> HHHHHHSEMTPREIVSELDKHIIGQDNAKRSVAIALRNRWRRMQLNEELRHEVTPKNILMIGPTGVGKTEIARRLAKLANAPFIKVEATKFTEVGYVGKEVDSIIRDLTDAAVKMVRVQAIEKNRYRAEELAEERILDVLIPPAKNNWGQTEQQQEPSAARQAFRKKLREGQLDDKEIEIDLAAAPMGVEIMA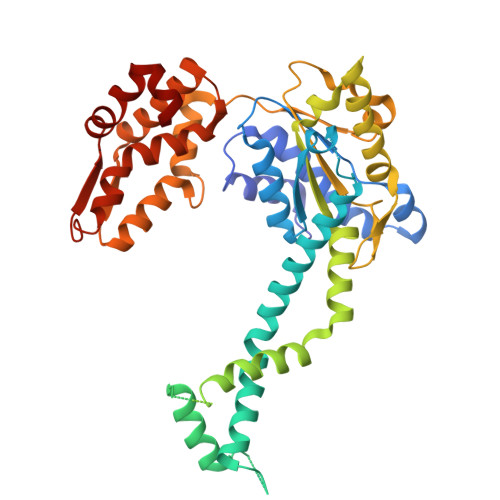PPGMEEMTSQLQSMFQNLGGQKQKARKLKIKDAMKLLIEEEAAKLVNPEELKQDAIDAVEQHGIVFIDQIDKICKRGESSGPDVSREGVQRDLLPLVEGCTVSTKHGMVKTDHILFIASGAFQIAKPSDLIPELQGRLPIRVELQALTTSDFERILTEPNASITVQYKALMATEGVNIEFTDSGIKRIAEAAWQVNESTENIGARRLHTVLERLMEEISYDASDLSGQNITIDADYVSKHLDALVADEDLSRFIL>MSAEGLDKDFCGAIIPDSFFPIEKLRNYTDMGIIREFAKGSAIIMPGED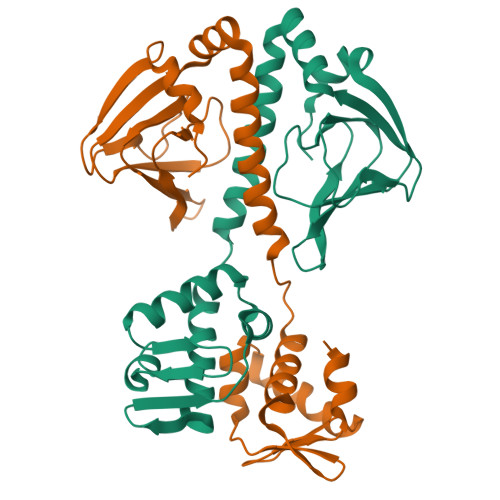TTSMIFLMDGKIKLDIIFEDGSEKLLYYAGSNSLIGRLYPTGNNIYATAMEQTRTCWFSEECLRVIFRTDEDMIFEIFKNYLTKVAYYARQVAEINTYNPTIRILRLFYELCSSQGKRVGDTYEITMPLSQKSIGEITGAHHVTVSKVLACLKKENILDKKKNKFIVYNLEELKHLSEQTSYY[2x]3-HYDROXY-5-(HYDROXYMETHYL)-2-METHYLISONICOTINALDEHYDE 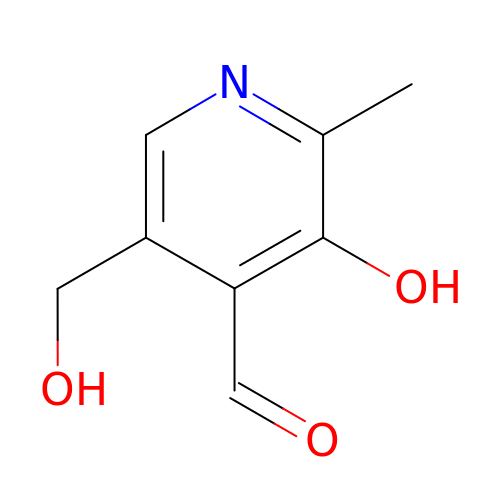| C8 H9 N O3 | RADKZDMFGJYCBB-UHFFFAOYSA-N>[2x]MLPQRLHPSRLLALALFSLVLGLAGCQTKPPQTGLSAEQIAVLQEQGFELRDEGWEFGMSSKVLFGNNLDRLNPDSRNTLTKIARALLAVDIDKVRLEGHTDNYGDEGYNQKLSERRAESVAAVFREAGMPAANIEVRGLGMSKPVADNKTRAGRSENRRVAIIVPAE

The tripartite signalling system YfiBNR in P. aeruginosa modulates intracellular c-di-GMP levels in response to signals received in the periplasm and is a key regulator of the SCV phenotype. The effector protein YfiN (also known as TpbB or PA1120) is an integral inner membrane protein that functions as a diguanylate cyclase, consisting of a periplasmic PAS domain, a cytoplasmic HAMP domain and a catalytic GGDEF domain. The third component of the YfiBNR signalling system, YfiR, has a key role in the signal transduction process by bridging YfiN in the inner membrane and YfiB in the outer membrane. YfiB can release the repression of YfiN by sequestering YfiR at the outer membrane, which requires both membrane anchoring and peptidoglycan binding by YfiB for full activity.

Crystal structures of the periplasmic domain of YfiB were determined for two different constructs: from residues 27–168 to 1.58 Å resolution, and from residues 59–168 to 1.39 Å resolution. The longer YfiB construct crystallizes with two molecules in an asymmetric unit while the shorter construct crystallizes with only one molecule per asymmetric unit. Analytical ultracentrifugation data confirms that YfiB(27–168) predominantly forms a dimer in solution, while YfiB(59–168) is exclusively a monomer. The structure of YfiB(27–168) is an OmpA-like domain with a core domain consisting of helices α1–3 and a four-stranded anti-parallel β-sheet with topology β1-β4-β2-β3 (following the numbering for the core conserved domain of Pal28). The N-terminal fragment visible from residues 30–53 includes an additional strand β1’ that packs anti-parallel to β1 in the core β-sheet, and helix α1’ that lies parallel to helix α2. The YfiB(27–168) structure reveals a weak asymmetric dimer whose interface buries approximately 421 Å2, or about 5.5% of the total surface area for each monomer, with a solvation free energy gain ΔG of −4.7 kcal mol−1 upon formation of the interface as calculated with PISA29. The predominantly hydrophobic dimer interface is formed by the N-terminal helix α1’ and strand β1’ of each monomer. The interfacing residues are mainly on helix α1’ and include Leu35, Ser36, Ala37, Glu38, Ile40, Ala41 and Gln44, with additional contributions from Phe48, Glu49 and Leu50 on strand β1’ and Trp55 on strand β1. Following superposition, it was evident that the N-terminal region of YfiB clashes considerably with YfiR, thus inhibiting the sequestration of YfiR. The weak dimer observed for YfiB(27–168) may help to suppress its role in YfiR sequestration by maintaining the linker in a folded conformation and thus inhibiting YfiR binding, although further experiments are required to confirm this.>MTYNVWNFGESNGRYSALTARGISKETCQKAGYWIAKVDGVMYQVADYRDQNGNIVSQKVRDKDKNFKTTGSHKSDALFGKHLWNGGKKIVVTEGEIDMLTVMELQDCKYPVVSLGHGASAAKKTCAANYEYFDQFEQIILMFDMDEAGRKAVEEAAQVLPAGKVRVAVLPCKDANECHLNGHDREIMEQVWNAGPWIPDGVVSALSLRERIREHLSSEESVGLLFSGCTGINDKTLGARGGEVIMVTSGSGMVMSTFVRQQALQWGTAMGKKVGLAMLEESVEETAEDLIGLHNRVRLRQSD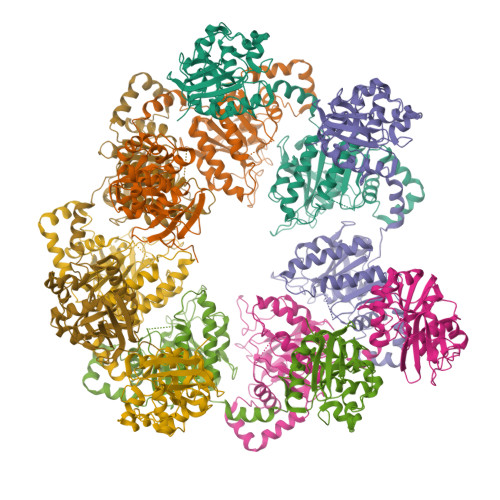SLKREIIENGKFDQWFDELFGNDTFHLYDSFAEAETDRLLAKLAYMRSGLGCDVIILDHISIVVSASGESDERKMIDNLMTKLKGFAKSTGVVLVVICHLKNPDKGKAHEEGRPVSITDLRGSGALRQLSDTIIALERNQQGDMPNLVLVRILKCRFTGDTGIAGYMEYNKETGWLEPSSYSGEEESHSESTDWSNDTDF[7x]>MSLKRKNIALIPAAGIGVRFGADKPKQYVEIGSKTVLEHVLGIFERHEAVDLTVVVVSPEDTFADKVQTAFPQVRVWKNGGQTRAETVRNGVAKLLETGLAAETDNILVHDAARCCLPSEALARLIEQAGNAAEGGILAVPVA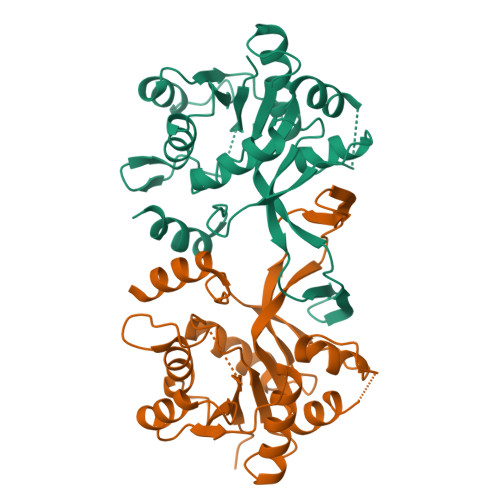DTLKRAESGQISATVDRSGLWQAQTPQLFQAGLLHRALAAENLGGITDEASAVEKLGVRPLLIQGDARNLKLTQPQDAYIVRLLLDAV[6x]> M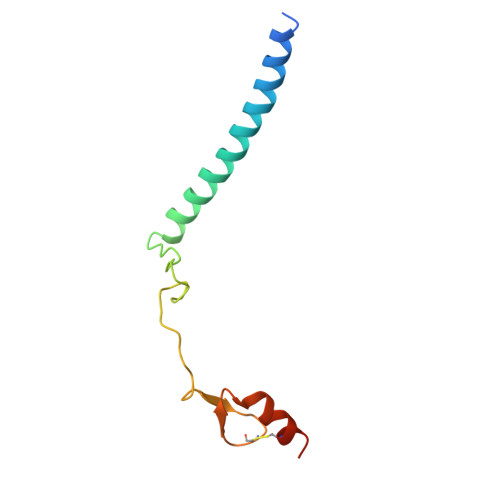TEETITIDSISNGILNNLLTTLIQDIVARETTQQQLLKTRYPDLRSYYFDPNGSLDINGLQKQQESSQYIHCENCGRDVSANRLAAHLQRCLSRGARR> LRYNLWFGVYDGKEIKLSENFEESFLKAENPSPLPFNVSEVGAKALGKDYYRILRKTALAVSEKMVEKELRREDRYVVALVKALEEIDESINMLNEKLEDIRAVKESEITEKFEKKIRELRELRRDVEREIEEVMEKIAPNMTELVGAKVAAKLLERAGSMERLVRLPASKIQVIGAEKSLYKAFARMKKGKKAKIPKHGIIFLHPFI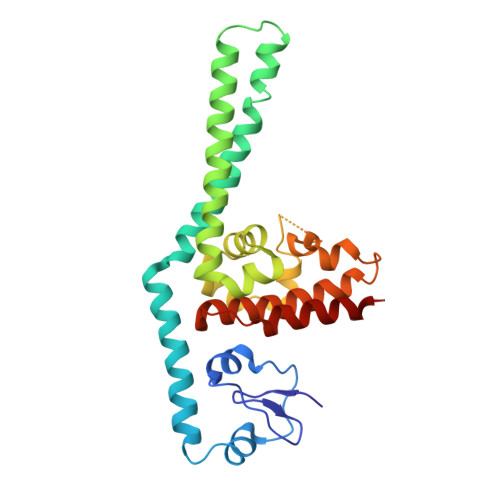RTLPKAKRGKMARFLAAKLAIAAKIDYFRGEIDESLYESIRRRYEELRRK(1S)-1-(4-fluorophenyl)-2-(1H-imidazol-1-yl)ethyl 3-(trifluoromethyl)benzoate | C19 H14 F4 N2 O2 | 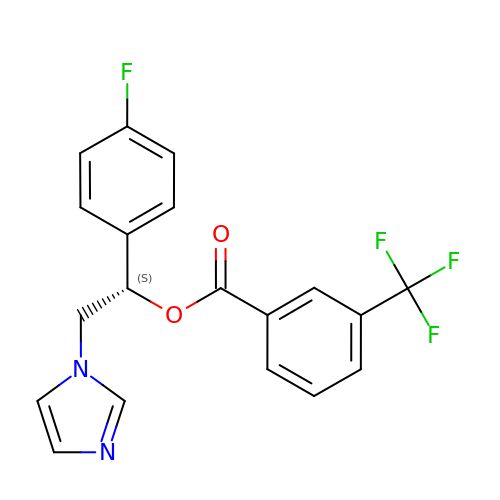FQDXUJLXGMFAIY-QGZVFWFLSA-N>AEEYGYIVTDQKPLSLAAGVKLLEILAEHVHMSSGSFINISVVGPALTFRIRHNEQNLSLADVT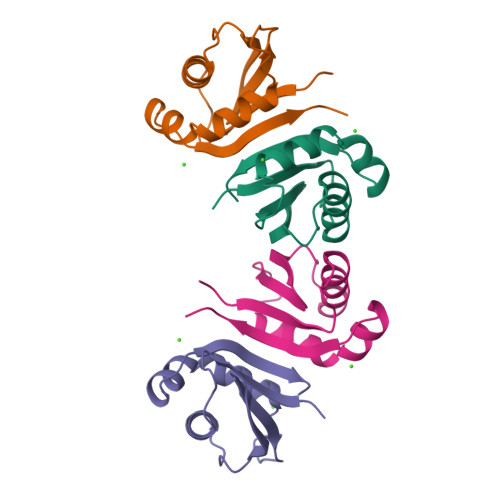QQAGLVKSELEAQTGLQILQTGVGQRE[2x]> SEPGKAHYFLAASGVDPGAAVRDLGALGLQAKTERTAASVGPAAG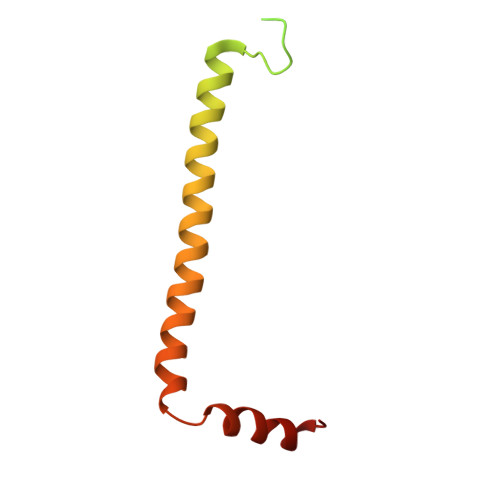PSGVSTTGFGTGLGEVDVDTYLSNLQTKTTLSMIADGLERSARDFDAFLEENVTLEWEAQRKRIYQHFGIK> ATIVALKYPGGVVMAGDRRSTQGNMISGRDVRKVYITDDYTATGIAGTAAVAVEFARLYAVELEHYEKLEGVPLTFAGKINRLAIMVRGNLAAAMQGLLALPLLAGYDIHASDPQSAGRIVSFDAAGGWNIEEEGYQAVGSGSLFAKSSMKKLYSQVTDGDSGLRVAVEALYDAADDDSATGGPDLVRGIFPTAVIIDADGAVDVPESRIAELARAIIESRSGADTFGSD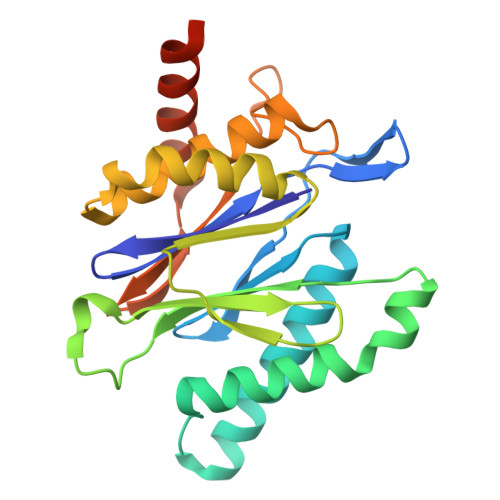GGEK> MQRIALSDKLELSRIVYGMWRIGDDADTSPAHVQAKIEACLAQGITTMDQADIYGGYTAEAILGGGLKAAPGLRDKIEIVTKCGIVAPAGRHSSA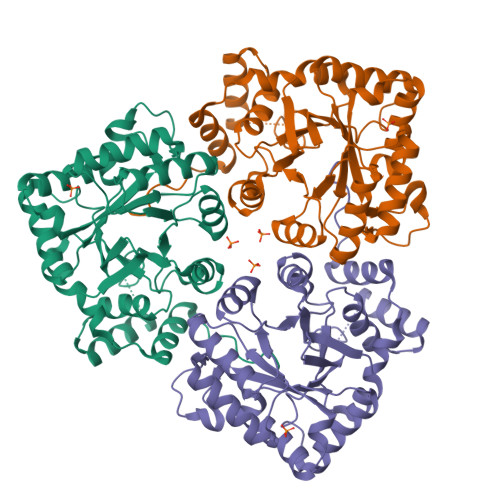RVKHYDTTAGHINVSVEASLRDMGTDHVDLLLIHRPDPLIDAEETGKALDALVASGKVKAVGVSNFRPWDFSLLQSAMSNRLVTNQIEMSLLATDTFTNGDLAYLQEKRVSPMAWSPLGGGSLFSGAYGGTMAALQRIGKEQGVDATAVAIAWLLRHPAKIVPVLGTNNLERIRTAADALRVTMDRQTWFELYTLAIGKEVALEHHHHHH Integration of retroviral DNA by the viral integrase (IN) into cellular DNA is a necessary step for virus replication. RSV IN is homodimeric in solution. The 3′ OH cleavage of blunt-ended viral DNA by IN yields intasomes with recessed ends, here termed the cleaved synaptic complex (CSC). We determined the structure of RSV octameric intasome stabilized by a HIV-1 IN strand transfer inhibitor using single particle cryo-electron microscopy.

The particles were grouped into five clusters (A–E) in their reaction coordinate space. The particles from each of these clusters were used to perform 3D reconstruction. We further refined these clusters by re-extracting the particles at maximum resolution and performed 3D reconstruction followed by homogeneous refinement. The refined structure for cluster E, with 64,449 particles, displayed the highest resolution (3.4 Å). The outer subunits in the proximal dimer have a relaxed conformation demonstrating an outward concerted movement of at least 5 Å when the distal NTD-CCD is further away from the CIC. When the distal NTD-CCD is closer to the proximal dimers, it makes the proximal dimers more compact. Comparison of the model generated with this refined cluster and the CSC intasome demonstrated the conformational heterogeneity in the distal subunits. These observations are consistent with a more relaxed CIC structure in the RSV CSC as compared to that in the STC, and highlights the overall dynamic potential of the RSV intasome.

>PLREAKDLHTALHIGPRALSKACNISMQQAREVVQTCPHCNSAPALEAGVNPRGLGPLQIWQTDFTLEPRMAPRSWLAVTVDTASSAIVVTQHGRVTSVAVQHHWATAIAVLGRPKAIKTDNGSCFTSKSTREWLARWGIAHTTGIPGNSQGQAMVERANRLLKDKIRVLAEGDGFMKRIPTSKQGELLAKAMYALNHFERGENTKTPIQKHWRPTVLTEGPPVKIRIETGEWEKGWNVLVWGRGYAAVKNRDTDKVIWVPSRKVKPDITQKDEVTKK[8x]> 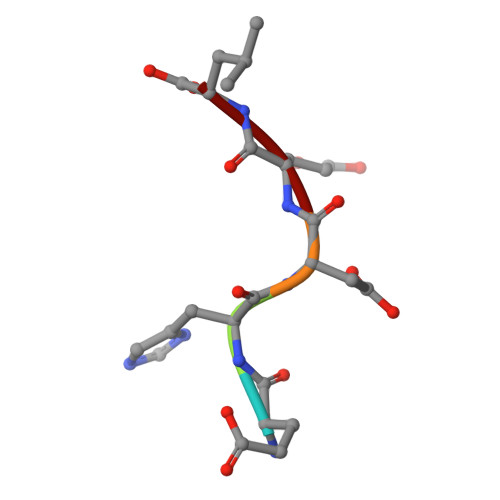EHDEL(2S)-3-(2-aminoethoxy)propane-1,2-diyl dihexadecanoate | C37 H73 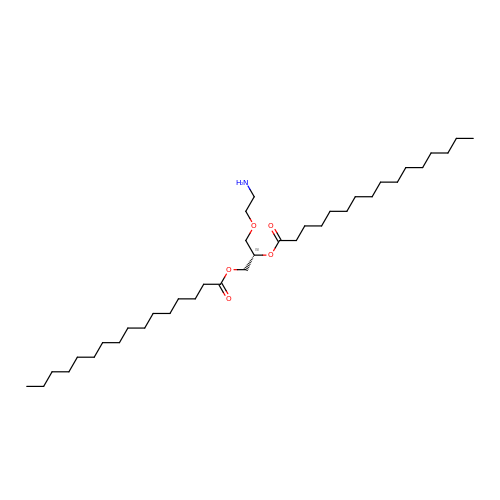N O5 | UWTLPHGXKLBELN-DHUJRADRSA-N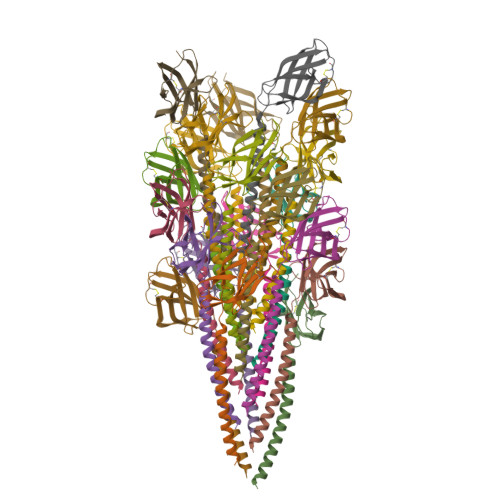>MPMKTKGLEPIVAAVLLIVVAVIGAVLVYLWFSGYVTRATSQAEQLSAAEQLKIEAVSKTGTTVSVNVRNVGEVPVKIASAYVLNATTLTMICGGSLTSPQQIDPGTIQTINVPGTCNLIAGARYIVKVVTARGTEAAATFISP[20x]> MPEYLSISKQKPDFPPYLNFQTLRDIGITHLQALSGKIWTDYNLHDPGVTILEVLCYAITDLGYRNNLDIADLLALNPQDGNSRENNFFTPDAVLTCNPVTELDVRKRLIDIPGVRNAWLQKVTSYEPNIYVNFSDKRLQYNPPTAESKTLNPRGLYTVRLDLDQDYRKNACGQIDRSWGDTLDEVKQVLCDSRNLCEDFADIVILGEEEIGICADIQLETNADAEDVLVNIYVRIQQFLSPRLKFYTLQELLDKGKSPAEIFAGRPSVFDGENRLYKSHGFIDTDELEALTLPTILHTSDLYQEILQVPGVSAIKKLSIANYINGLRQTQGHPWYLQLTDQYRPVLGVKTSKINFFKSELPIGVDEEEVERRY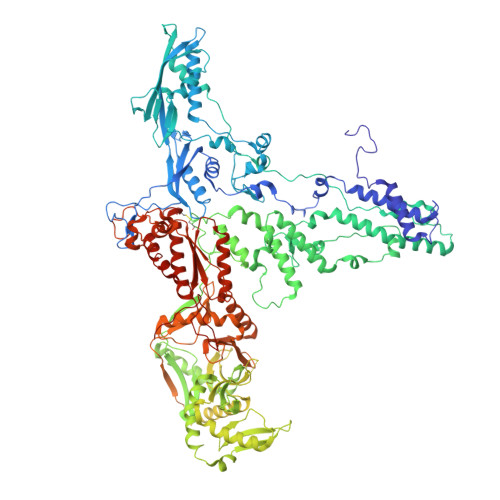YEQQAAYIKTIRDRDELDIPVPKGSYYDLADHYSIHHDFPTTYGISEDGLPPTVPALRKAQALQLKAYLVFFDQLLASYLAQLSHIRDLFSWEVDVTQPQQNDYATRLQEKQRTYFTQKLDFPEIEKIIPDNYLDVLDEAPETYRDRRNRFLDHLLARFSESFSDYVLLNYQMFATRNNKATQETEIIHDKAQFLQDYPTLSRDRFRAYNYYDCHAVWDTDNVAGFKKRVLRLLGIDDVRRRHLSHYRVDKDSRNLFLSIDFSSDDLTLTSKQRYATTEQAQADQDKLLLFALHPNFYKRLSYKYYYHYSWEILDTQNQSIVRSDRFFPSTKERAAALEPLLQSLLTQLSQLDDTALQNLVITQPTDEDLYSFRLQIPLNSGVITFTGVQRYFSRTEAVDAGVISLRLIQDVQNYRNITLGQDQGTTPQKFTYYGYGLVDHQGSLLSEYTHHFPTELERELSLQRWLTHIQANQNQYKFAIETITNGYVFVINDITNSQTLLRGISSYATEYLAWQAASEFAENLRYLNRYLSPAKDHTGQTYSLGITDKTGKLLAVTTTESDRLLTFQRLNALEPFLVIEAATTPTSGYRYRLVDRQETTILQSIQIYGDETTARDRFYQDVLGTLFETGVINPTTTNKEFGFRILSRPRDTNSVAAIHTQTYTSEAERDAAIEHLLLLVRTARLRISTNSLDSLAYISQIYNPDNQLILQGTQRYTSEDIAWEQGNTLMELAQDEENFRLIDSDDGVYGWELTNEGKDEIFAAQYYNSREERTAAIAEIQKYSNDEGFHLLEHILLRPRTKLPDLTAGDGFLPILVTPEDVNTEPDDPYLLARTDPYSFWVTIVLPYWPQRFRDIPFRRFVERTLRLEAPAHIALKIAWVNVRQMRDFELAYRHWLEQLALESCENAACDLTGTLNRLLKILPQLRNVYPKATLHDCEESSADNNPAILNQTALGTAND> AAAYWDCDGTEIPERNVRAAVVLAFNYRKESFHGYPATFIIGSTFSGVGEVRQFPVEDSDANWQGGAVKYYILTNKRGSYL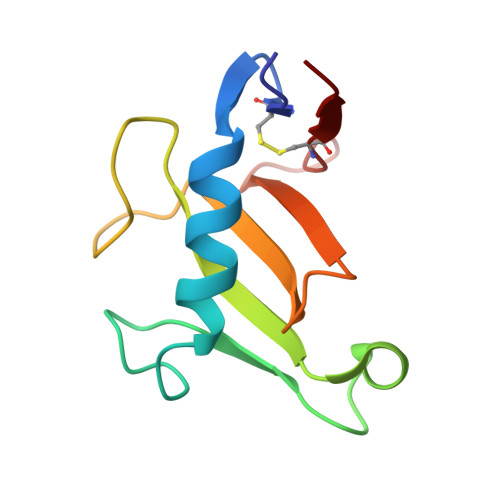EVFSSVGSGNKCTFVEG4-methyl-2-(4-methylphenyl)-5-(1H-pyrazol-5-yl)-1,3-thiazole | C14 H13 N3 S | 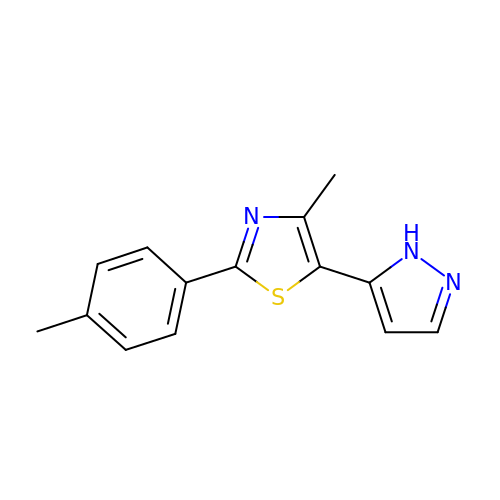OWUYIJUAGSAJFL-UHFFFAOYSA-N>[4x]SFTMTWLPLNPIPLKDRVSMIFLQYGQIDVIDGAFVLIDKTGIRTHIPVGSVACIMLEPGTRVSHAAVRLAAQVGTLLVWVGEAGVRVYASGQPGGARSDKLLYQAKLALDEDLRLKVVRKMFELRFGEPAPARRSVEQLRGIEGSRVRA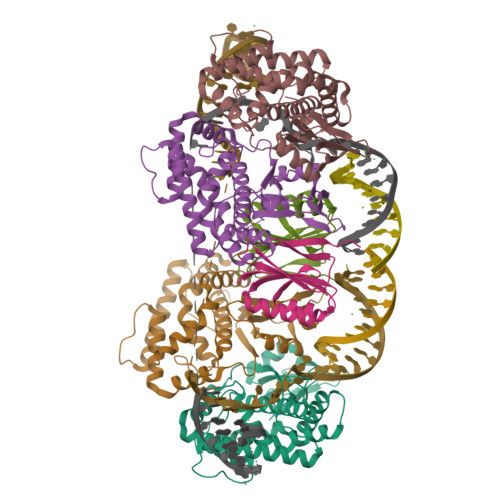TYALLAKQYGVTWNGRRYDPKDWEKGDTINQCISAATSCLYGVTEAAILAAGYAPAIGFVHTGKPLSFVYDIADIIKFDTVVPKAFEIARRNPGEPDREVRLACRDIFRSSKTLAKLIPLIEDVLAAGEIQPPAPPEDAQPVAIPLPVSLGDAGHRSS;>[2x]MSMLVVVTENVPPRLRGRLAIWLLEVRAGVYVGDVSAKIREMIWEQIAGLAEEGNVVMAWATNTETGFEFQTFGLNRRTPVDLDGLRLVSFLPVGSSENLYFQ> MSYSAYFAKAGFQFPAGLSALVAGIVALNVCTGRPTKGTKEISNAEYNATPIGYLQSPDQHPTAFPKVPGMKDVHGSPHHHH;> MMRAAQKAKQELPATVLTQTRSYLAPLRSDFTEEITAPKVASASNLVNEWNNKKQATENLMKLLQAYKDIGDAKSEPLLKNHNPRTFEDRDYPVPDFRTQNLKAGDVPKFFDTVISTRASAAIASKDKFWAGRKTEAEAASAKASAAFPRVAVPEWKKGKTVSIENLNTVTDKYAAALVPKRKLALPVLPEGVKKAVEDFAASVGQAKNASEVSELLAKSLAEKAVVTEGGKVVEGFSYVSKAVAAKVIATRRAEVHERLLKLWAKRLLVSPELAIVPLNEFDAQLASKFEGISPKYQELLSAVAQGNKTFAQRLNSSPAFSSFLLKREKAESEVPPSELELEAAQKAAELEDPEVALRTLLGPQMEALGASDLLLSEQIRVITEHRYTPDRLQYKEGMKLADKIAAQEAALKEELKVIYGDNVDVKHFQASPRTPVQQLFDSLKNAAANKERAAKEAAAAASPYLAYAVTKKQEVQADPSNIPFDEVLYPQLSEELLELELSDIREDEIALEKAEEEELWLLTLTQQFKHIQKHFGIDLPHSVVAHMDPLLIKKIDWETTNALEDFDITLDDMGAEDAKEQWGAENLSHHFLPLIRYRRDLARKNGDRYGPDLVNGN;> MRQASRLALSIRQAGNVEAASAVPAMTRQFSAPGSHEHHETPLSKVMPTVVSIPRKVACLALGATKKVVCGLASSGPSQNLVSTFANKVIVEENLVNVAEIDVPFWSYWLSSAGFTSKDAFVKFAEAVKPKVAALSTSDITNLTVAFKRANYYDKDLFTGIEANVSANFTKFETEQLLQIVATFDAFNHSSVAFLDDVADSITYCNHYLAPVRAGADELATLLTYYAKNGHERADLLATVARGFSEVSLGKLSAAQRKDTVLSALKAFQTFGFYPESIEAVIGAALVSPAEYSAEELKEVEAVKVAAENALGGEFVLIQEGAHGH;> MKLLPESLQQEAATAAVVASWVLWHLDTQLLPTIMREHKLHACWAAAAKRYNEKLFKLNPSYDRVLSLPAVSKNQVLENVFHTAPKAPVEHLEKMVSANSKVYDALNLQSKRVLIWQVKPALF;> MMLRTLTRSSAVAGQAVRLFKTSAAAAEGNSVAGIIKSVNETSGANLLSSLKTIKAQAAPIYPAAASSTGYSTQAKIALFGALSWILYRADGQSKAHEWIVDLNLNVLQAAWLISFSSLIPFRAVYFAFRGMAPATASTLNGLKTFSSISL;> MSSVRAGVEAGRRDLTTFTFSGLQDAPVAALSGSIKLNVAAKAGKAEVTVAAGAAKAATQVSAAALRKLSGSKISLAEVARISVLHSSIQNYLLSLSNERYQLLSQWPDFTTMYGKDFYYRAHPEDLKKFYDAADEYYKLYETVTEFDSLSALASQVVPNYAARRRSTVHPAIGSTVADGAFTNFLLSKQ;> MVLGEVYLKDILRTPPTGAIPANVPHPFQTSFYTYATKKLIPRHWYLLGGFTFTITLYGILDGLRDSGKKKAYDEAIHAGKTPYTAGGH;> MAVTSFLGKAFEKYFYDFSAYEQFGLNRFLSSKGQYVALRHVGFVMVGVNVLLAANFPFNPPFPTIGMCPAGWEGTWVCQADKAKALEMYKEWKKSN;> MSVLSSVSMGSRIGSSLLGRSSAYLAQCGFSTRSNLNGSIDTSSSVFQALSSDNENKPAASPLNVKLPGMSCSSILLPKTSRIAVPFGNQTMAMSSVRDVKTGSLPTNFLTGVYRFWRSQNPAEKPHDPVNDRLLPAVVDASDKRASIGTWATTFFCTIISCNLLGLMPFNEAPTSGLGFATGLGVSVWATATILGLSKTGFKFPGHFIPGGTPWPMAFIFVPLETISYTFRAVSLGVRLWVNMLAGHTLLHILTGMALALPF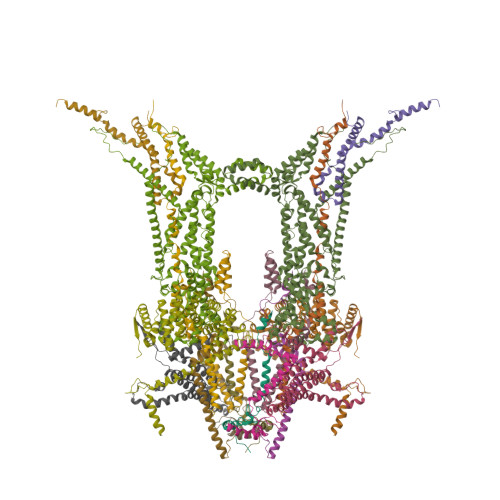SLGFFSMVPATFGVCCLLSALVGLEYLVAVLQSGVFSILSTVYVGEFNHDKFIGPAAKIVKKIH Langya virus (LayV) was recently found in shrews and isolated from febrile patients in China, representing the first human-infecting HNV from shrew origin. HNV infections are facilitated by the attachment glycoprotein (G) and the fusion glycoprotein (F). Upon G-mediated receptor engagement, F is triggered and promotes membrane fusion and viral entry. LayV F and G are closely related to MojV F and G but distantly related to their NiV and HeV counterparts.

Computational design of optimal residue replacements were aided by ProteinMPNN and visually inspected to generate LayV GSM, comprising the F89L, G98T, G117A, F126V, and Y130L substitutions. To unveil the 3D organization of LayV G, we determined a 3.2 Å resolution cryoEM structure of LayV GSM fused to a designed tetramerization motif (designated oP4h) at its N-terminus. LayV G folds as a 150 Å-high and 140 Å-wide fourfold symmetrical tetramer with a central stalk surrounded by four β-propeller head domains. The stalk region built in the cryoEM density comprises residues 68 to 142 and the β-propeller head domain comprises residues 176 to 607. Residues 166 to 175 of the intervening linker region mediates interprotomer interactions with a neighboring head domain. The four LayV G head domains form a fourfold symmetrical clamp around the central stalk with each β-propeller interacting with two neighboring heads and with the stalk helices from two distinct protomers. The LayV G head domain conformation observed in our structure differs from that found in NiV G, as the latter glycoprotein adopts an asymmetric organization of its head domains with only two of them interacting with the stalk. The observed LayV G head conformation and symmetry are unique among characterized paramyxovirus attachment glycoproteins. The stalk is a four-helix coiled coil with intervening pi-helices at residues 97 to 101 and 111 to 115 mediated by prolines at residues 102 and 116, consistent with the NiV G stalk. Approximately twenty additional residues could be resolved at the N-terminal region of the stalk, relative to the NiV G structure, revealing a 310-helix at residues 86 to 89.

>[4x]MTRLTVLALLAGLLASSRASGPHHHHHHHHGSSPQAEELKAIKEELKAIKEELKAIKEELKAIQAMLKIIQDEVNSKLEMLVSLDQLVKTEIKPKVSLINTAVSVSIPAQISNLQTKVLQKLVYLEESITKQCTCNPLSGIFPTTKPPPPPTDKPDDDTTDDDKVDTTIKPVEYYKPDGCNKTNDHFTMQPGVNFYTVPNLGPSSSSADECYTNPSFSIGSSIYMFSQEIRKTDCTTGEILSIQIVLGRIVDKGQQGPQASPLLVWSVPNPKIINSCAVAAGDETGWVLCSVTLTAASGEPIPHMFDGFWLYKFEPDTEVVAYRITGFAYLLDKVYDSVFIGKGGGIQRGNDLYFQMFGLSRNRQSIKALCEHGSCLGTGGGGYQVLCDRAVMSFGSEESLISNAYLKVNDVASGKPTIISQTFPPSDSYKGSNGRIYTIGERYGIYLAPSSWNRYLRFGLTPDISVRSTTWLKEKDPIMKVLTTCTNTDKDMCPEICNTRGYQDIFPLSEDSSFYTYIGITPSNEGTKSFVAVKDDAGHVASITILPNYYSITSATISCFMYKEEIWCIAVTEGRKQKENPQRIYAHSYRVQKMCFNIKPASVVTSLPSNVTIRS> S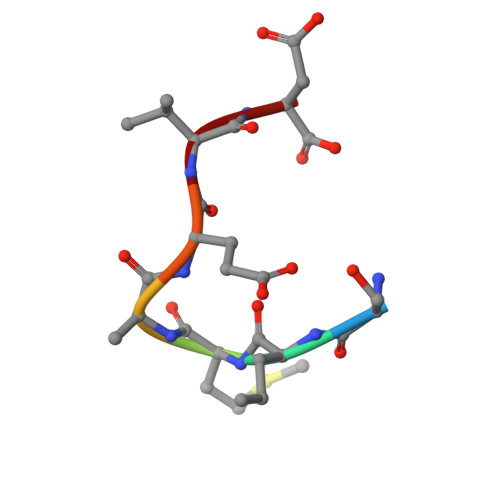RMEEVD> KPCDLPLRLLVPTQFVGAIIGKEGATIRNIT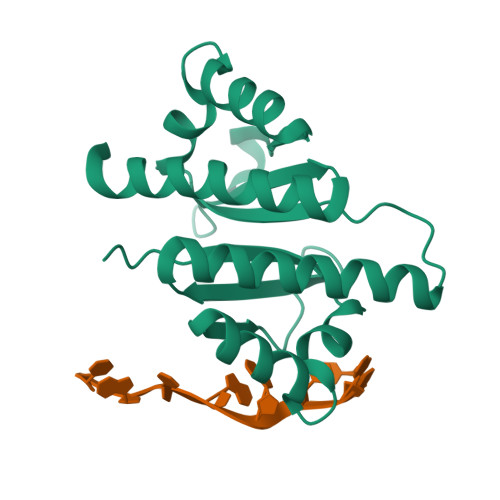KQTQSKIDVHRKENTGAAEKSITILSTPEGTSAACKSILEIMHKEAQDIKFTEEIPLKILAHNNFVGRLIGKEGRNLKKIEQDTDTKITISPLQELTLYNPERTITVKGSVETCAKAEEEIMKKIRESYENDI>[2x]SQKLDDVDPLVTTNFGKIRGIKKELNNEILGPVIQFLGVPYAAPPTGEHRFQPPEPPSPWSDIRNATQFAPVCPQNIIDGRLPEVMLPVWFTNNLDVVSSYVQDQSE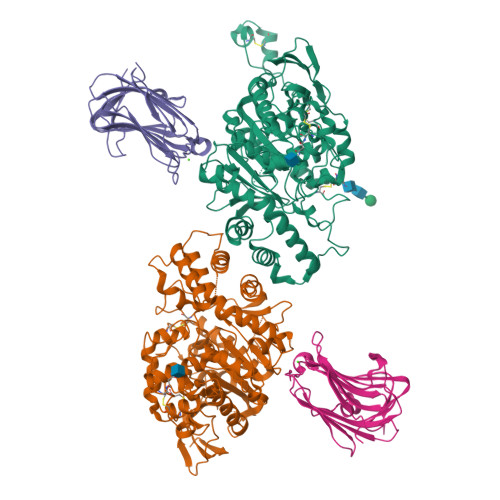DCLYLNIYVPTEDVKRISKECARKPGKKICRKGDIRDSGGPKPVMVYIHGGSYMEGTGNLYDGSVLASYGNVIVITVNYRLGVLGFLSTGDQAAKGNYGLLDLIQALRWTSENIGFFGGDPLRITVFGSGAGGSCVNLLTLSHYSEGLFQRAIAQSGTALSSWAVSFQPAKYARILATKVGCNVSDTVELVECLQKKPYKELVDQDVQPARYHIAFGPVIDGDVIPDDPQILMEQGEFLNYDIMLGVNQGEGLKFVENIVDSDDGVSASDFDFAVSNFVDNLYGYPEGKDVLRETIKFMYTDWADRHNPETRRKTLLALFTDHQWVAPAVATADLHSNFGSPTYFYAFYHHCQTDQVPAWADAAHGDEVPYVLGIPMIGPTELFPCNFSKNDVMLSAVVMTYWTNFAKTGDPNQPVPQDTKFIHTKPNRFEEVAWTRYSQKDQLYLHIGLKPRVKEHYRANKVNLWLELVPHLHNLND;>[2x]GSGTTYIFSKGGGQITYKWPPNDRPSTRADRLAIGFSTVQKEAVLVRVDSSSGLGDYLELHIHQGKIGVKFNVGTDDIAIEESNAIINDGKYHVVRFTRSGGNATLQVDSWPVIERYPAGRQLTIFNSQATIIIGGKEQGQPFQGQLSGLYYNGLKVLNMAAENDANIAIVGNVRLVGEVS4-tert-butyl-N-(1,3-diphenyl-1H-pyrazol-5-yl)benzamide 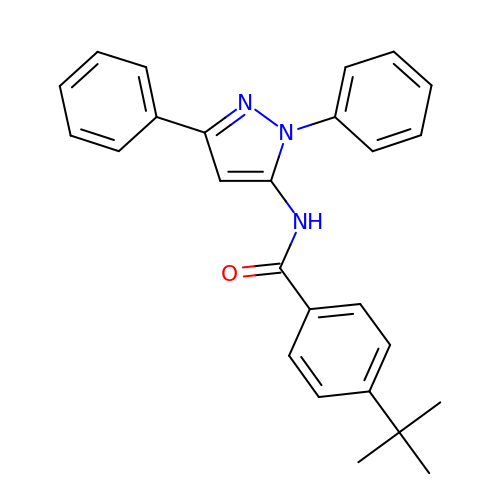| C26 H25 N3 O | GTSXKUJFTQTICP-UHFFFAOYSA-N> GSHMSRKIRDLIESKRFQNV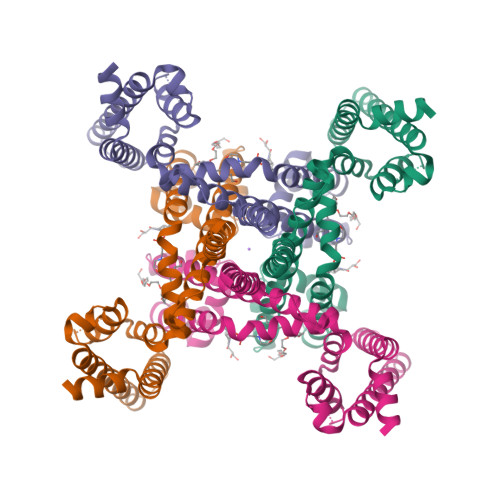ITAIIVLNGAVLGLLTDTTLSASSQNLLERVDQLCLTIFIVEISLKIYAYGVRGFFRSGWNLFDFVIVAIALMPAQGSLSVLRTFRIFRVMRLVSVIPTMRRVVQGMLLALPGVGSVAALLTVVFYIAAVMATNLYGATFPEWFGDLSKSLYTLFQVMTLESWSMGIVRPVMNVHPNAWVFFIPFIMLTTFTVLNLFIGICVDAMAITKEQEEEAKTGHHQEPISQTLLHLGDRLDRIEKQLAQNNELLQRQQPQKK>MAHHHHHHMLDLANRFNFEGHRIAWGTLGEGPPLVLVHGTPFSSQVWRRIAPWLARRHRVFFYDLLGYGQSDMPDADVSLGRQ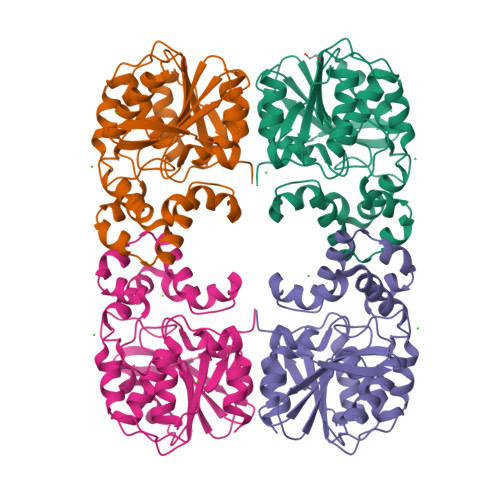NVLFGALLDEWKISRPRVLAHDYGGATVLRAHFLDGIAYSDLTLVNPVAIAPQGSPFVRHVAQHEAAFTGLPAYAHHALVSAYIGQAVAQPLSDDVLSIYRAPWLTPAGQAAFYRQIAQMRQRYIEDAEARYAPPDFPVRIVWGEDDRWIPLEQGQALADRIANGKLIRVPRAGHLVQEDAPEAIVAAVLDR[4x]>MTMDEQQSQAVAPVYVGGFLARYDQSPDEAELLLPRDVVEHWLHAQGQGQPSLSVALPLNINHDDTAVVGHVAAMQSVRDGLFCLGCVTSPRFLEIVRRASEKSELVSRGPVSPLQPDKVVEFLSGSYAGLSLSSRRCDDAEAPTSLSGSETTPFKHVALCSVGRRRGTLAVYGRDPEWVTQRFPDLTAADRDGLRAQWQRCGSTAVDASGDPFRSDSYGLLGNSVDALYIRERLPKL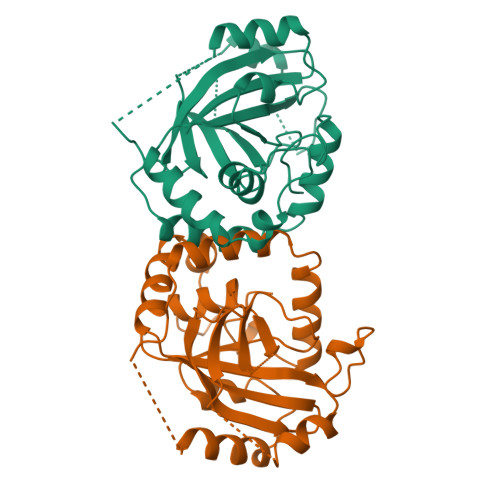RYDKQLVGVTERESYVKA[2x]> MIKVEIKPSQAQFTTRSGVSRQGKPYSLNEQLCYVDLG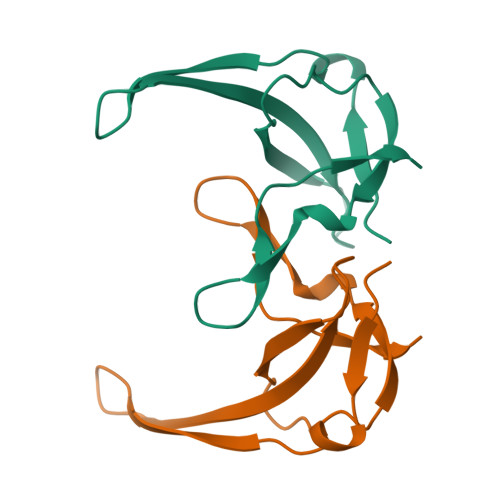NEYPVLVKMTLDEGQPAYAPGLYTVHLSSFKVGQFGSLMIDRLRLVPAK2-(5-chlorothiophen-2-yl)-N-{(3S)-1-[3-fluoro-2'-(methylsulfonyl)biphenyl-4-yl]-2-oxopyrrolidin-3-yl}ethanesulfonamide 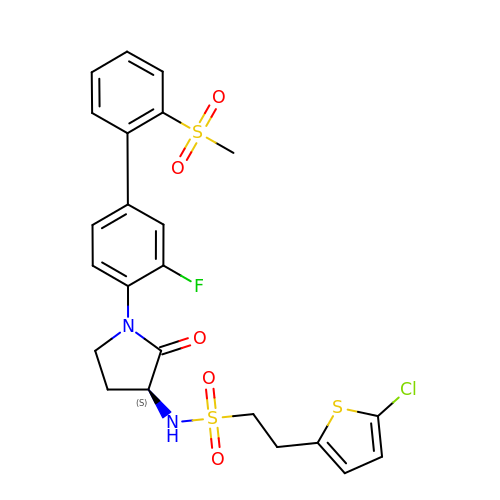| C23 H22 Cl F N2 O5 S3 | MRKBPFVJGAHTFU-IBGZPJMESA-N> MAMPFEIEVLLPGELSPAETSALQKCEGKIITFSTLRHRASLVDIALSSYYINGAPPDTLSLLEAYRMRFAAVITRVIPGKLLAHAIGVGTPTPGLFIQNTSPVDLCNGDYICLLPPVFGSADSIRLDSVGLEIVFPLTIPQTLMREIIAKVVARAVERTAAGAQILPHEVLRGADVIC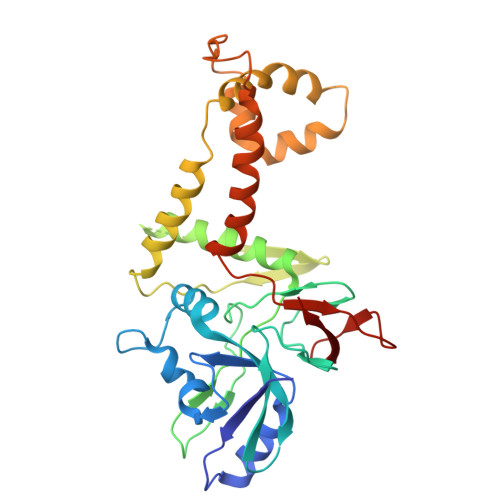YNGRRYELETNLQHRDGSDAAIRTLVLNLMFSINEGCLLLLALIPTLLVQGAHDGYVNLLIQTANCVRETGQLINIPPMPRIQDGHRRFPIYETISSWISTSSRLGDTLGTRAILRVCVFDGPSTVHPGDRTAVIQV>CGCTCTAGAGCG[4x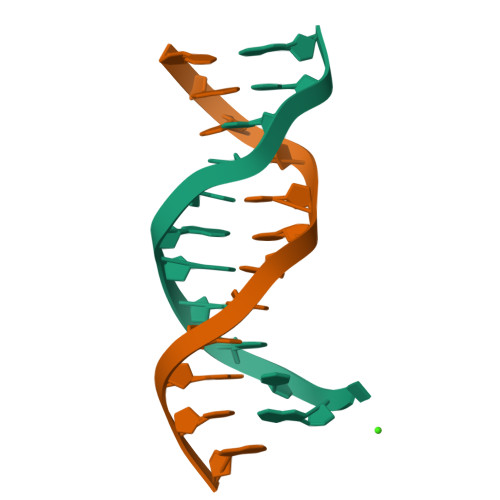]>MVDPATLSKLEAGFQKL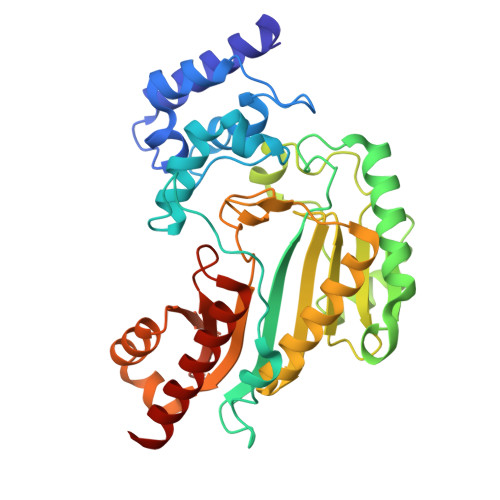QNAQDCHSLLKKYLTRDVFDQLKNKKTDMGATLLDVIQSGVENLDSGVGIYAPDAQSYKTFAALFDPIIDDYHKGFKPTDKHPKTDFGNIENFVNVDPKNEYVLSTRVRCGRSLNGYPFNPMLTEAQYKEMETKVKGQLATFEGELKGTYYPLLGMDKATQQQLIDDHFLFKEGDRFLQAANACRYWPVGRGIFHNDKKTFLMWVNEEDHLRIISMQKGGDLKEVYGRLVKAVKHIEQKIPFSRDDRLGFLTFCPTNLGTTIRASVHIKLPKLAADRKKLEEVAGRYNLQVRGTAGEHTESVGGIYDISNKRRMGLTEYQAVKEMQDGILELIKMEKSM[2x]> MEKNID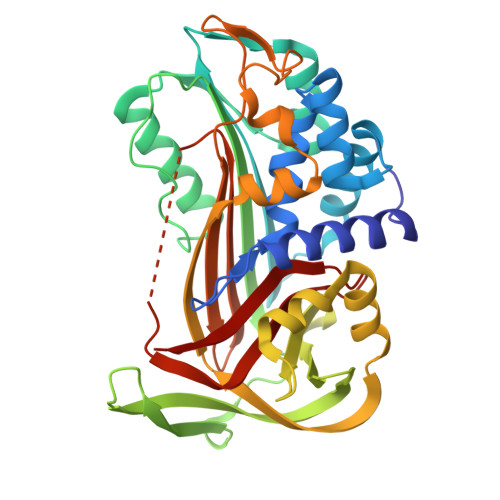EKFIYNTADFSIELFKNSIDDKENSLISPLSAMLALAMTANGADNETLAQMEKALGKDISIEDLNKYLYTYMKKLPNEEKSKLTIANSIWFKENDFMPSKDFLQIIADYYKADIFKAAFDSSTVSDINNWVKSKTNGMIDKILNKIDPEDVMYLINAVAFDAEWETVYEKASVHEDIFTDVYGNRQKVEFMNSEENLYIEEENAVGFVKPYAKNHYSFVAILPDENISVNEYIKTLTGQKFIDLIKNAKITLVRASLPKFKYEYTIKMNETLESLGMTDAFLPDKADFSKLGKSDIGNLYISEVLHKTFISVDELGTKAGAVTSVDITAAGIPVNFKTVKLNRPFIFAIIDNSTNLPIFIGTVLSLK>[15x]GDEMVTRVVPVRNVSVRELAPLLRQLNDNAGGGNVVH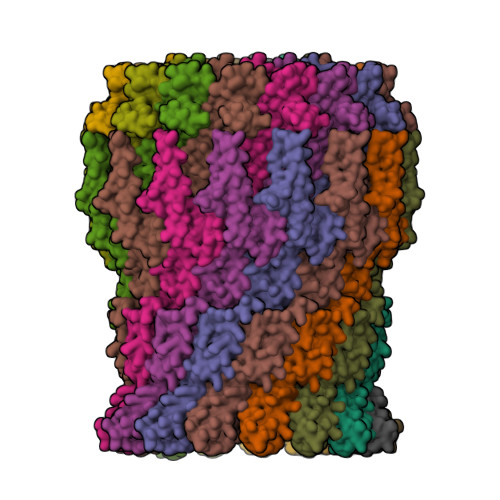YDPSNVLLITGRAAVVNRLVEVVRRVDKAGDQEVDIIKLKYASAGEMVRLVTNLNKDGNSQGGNTSLLLAPKVVADERTNSVVVSGEPKARARIIQMVRQLDRELQSQGNTRVFYLKYGKAKDMVEVLKGVSSSIEADKKGGGTATTAGGGASIGGGKLAISADETTNALVITAQPDVMAELEQVVAKLDIRRAQVLVEAIIVEIADGDGLNLGVQWANTNGGGTQFTNAGPGIGSVAIAAKDYKDNGTTTGLAKLAENFNGMAAGFYQGNWAMLVTALSTNTKSDILSTPSIVTMDNKEASFNVGQEVPVQTGTQNSTSGDTTFSTIERKTVGTKLVLTPQINEGDSVLLTIEQEVSSVGKQATGTDGLGPTFDTRTVKNAVLVKSGETVVLGGLMDEQTKEEVSKVPLLGDIPVLGYLFRSTSNNTSKRNLMVFIRPTILRDANVYSGISSNKYTLFRAQQLDAVAQEGYATSPDRQVLPEYGQD>[12x]MAETLEKKHERIMLRFDRAYSPQKEVREKCIEATRFARVPGGQWEGATAAGTKLDEQFEKYPKFEINKVATELNRIIAEYRNNRITVKFRPGDREASEELANKLNGLFRADYEETDGGEACDNAFDDAATGGFGCFRLTSMLVNEYDPMDDRQRIAIEPIYDPSRSVWFDPDAKKYDKSDALWAFCMYSLSPEKYEAEYG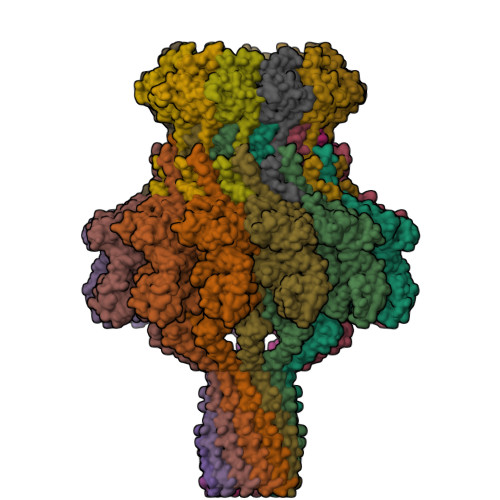KKPPTSLDVTSMTSWEYNWFGADVIYIAKYYEVRKESVDVISYRHPITGEIATYDSDQVEDIEDELAIAGFHEVARRSVKRRRVYVSVVDGDGFLEKPRRIPGEHIPLIPVYGKRWFIDDIERVEGHIAKAMDPQRLYNLQVSMLADTAAQDPGQIPIVGMEQIRGLEKHWEARNKKRPAFLPLREVRDKSGNIIAGATPAGYTQPAVMNQALAALLQQTSADIQEVTGGSQAMQQMPSNIAQETVNNLMNRADMASFIYLDNMAKSLKRAGEVWLSMAREVYGSEREVRIVNEDGSDDIAVLSAQVVDRQTGAVVALNDLSVGRYDVTVDVGPSYTARRDATVSVLTNVLSSMLPTDPMRPAIQGIILDNIDGEGLDDFKEYNRNQLLISGIAKPRNEKEQQIVQQAQMAAQSQPNPEMVLAQAQMVAAQAEAQKATNETAQTQIKAFTAQQDAMESQANTVYKLAQARNIDDKAVMEAIRLLKDVAESQQQQFQSPPQSPADLMPS;>[12x]MATVLTKGEIVLFALRKFAIASNASLTDVEPQSIEDGVNDLEDMMSEWMINPGDIGYAFATGDEQPLPDDESGLPRKYKHAVGYQLLLRMLSDYSLEPTPQVLSNAQRSYDALMTDTLVVPSMRRRGDFPVGQGNKYDVFTSDRYYPGDLPLIDGDIPNA>[3x]MMGNKLTLPAELPDEQDLRAVLAYNMRLFRVNKGWSQEELARQCGLDR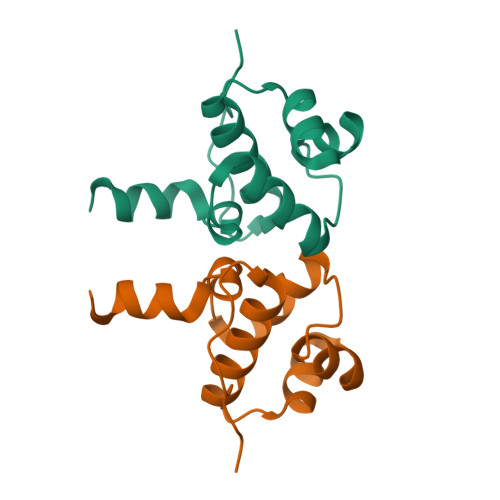TYVSAVERKRWNIALSNIEKMAAALGVAAYQLLLPPQERLKLMTNSADTRQMPSESGILEHHHHHH Epstein-Bar virus (EBV), a member of the subfamily gammaherpesviruses that also includes the Kaposi Sarcoma-associated herpesvirus (KSHV),2,3 is the first identified oncovirus. Similar to other members of the family herpesviridae, EBV has a characteristic three-layer configuration: the outer lipid bilayer envelope containing viral glycoproteins responsible for host recognizing and membrane fusion, the inner pseudo-icosahedral nucleocapsid enclosing a 172-kb double-strand DNA (dsDNA) genome and the middle pleomorphic tegument compartment fulfilled with 20–40 different viral proteins. All herpesvirus capsid shell consists of 4 abundant proteins: the major capsid proteins (MCP) constituting the basic capsid skeleton through forming 150 hexons and 11 pentons, the small capsid proteins (SCP) binding to the tops of hexon MCPs or both hexon and penton MCPs, and the Tri1 and Tri2 forming the heterotrimeric triplexes to plug the large holes on the capsid floor. Once the viral dsDNA genome enters the procapsid shell through the portal that is located at a unique 5-fold vertex of the icosahedral capsid, the viral nucleocapsid is joined by the capsid-associated tegument complexes (CATCs).

We also determined the high-resolution structure of the CATC in portal-proximal penton vertices where the CATC binds exclusively to a specific one of the five registers. In order to do so, we performed focused 3D classification of the portal-proximal penton-vertex sub-particles (extracted from the C1 capsid) with a mask encompassing a region containing only one CATC. We finally obtained 93,334 (83.3%) CATC-binding portal-proximal penton vertex sub-particles. Through 3D refinement, we obtained reconstruction of the C1 CATC-binding portal-proximal penton vertex at 4.3 Å. The structure of CATC in the portal-proximal penton vertex is essentially identical to that in the portal vertex. Unlike its counterpart in KSHV that interacts with only one MCP,22 the head domain of BVRF1 simultaneously contacts two neighboring penton MCPs, mainly through the region of residues 291–314. As such, pORF64 (the BVRF1 homolog in KSHV) interacts with one penton MCP at the apex, whereas the head domain of EBV BVRF1 simultaneously contacts two neighboring MCPs at the middle of the MCP tower region. Each CATC binds both triplexes Ta and Tc. The interactions between the CATC and Ta are exclusively mediated by BGLF1. The interactions between the CATC and triplex Tc occur at the vertex-distal end of the CATC.

>MARRLPKPTLQGRLEADFPDSPLLPKFQELNQNNLPNDVFREAQRSYLVFLTSQFCYEEYVQRTFGVPRRQRAIDKRQRASVAGAGAHAHLGGSSATPVQQAQAAASAGTGALASSAPSTAVAQSATPSVSSSISSLRAATSGATAAASAAAAVDTGSGGGGQPHDTAPRGARKKQ[5x];>MKVQGSVDRRRLQRRIAGLLPPPARRLNISRGSEFTRDVRGLVEEHAQASSLSAAAVWRAGLLAPGEVAVAGGGSGGGSFSWSGWRPPVFGDFLIHASSFNNAEATGTPLFQFKQSDPFSGVDAVFTPLSLFILMNHGRGVAARVEAGGGLTRMANLLYDSPATLADLVPDFGRLVADRRFHNFITPVGPLVENIKSTYLNKITTVVHGPVVSKAIPRSTVKVTVPQEAFVDLDAWLSGGAGGGGGVCFVGGLGLQPCPADARLYVALTYEEAGPRFTFFQSSRGHCQIMNILRIYYSPSIMHRYAVVQPLHIEELTFGAVACLGTFSATDGWRRSAFNYRGSSLPVVEIDSFYSNVSDWEVIL[2x];>MDLKVVVSLSSRLYTDEIAKMQQRIGCILPLASTHGTQNVQGLGLGQVYSLETVPDYVSMYNYLSDCTLAVLDEVSVDSLILTKIVPGQTYAIKNKYQPFFQWHGTGSLSVMPPVFGREHATVKLESNDVDIVFPMVLPTPIAEEVLQKILLFNVYSRVVMQAPGNADMLDVHMHLGSVSYLGHHYELALPEVPGPLGLALLDNLSLYFCIMVTLLPRASMRLVRGLIRHEHHDLLNLFQEMVPDEIARIDLDDLSVADDLSRMRVMMTYLQSLASLFNLGPRLATAAYSQETLTATCWLR[4x];>MSNGDWGQSQRTRGTGPVRGIRTMDVNAPGGGSGGSALRILGTASCNQAHCKFGRFAGIQCVSNCVLYLVKSFLAGRPLTSRPELDEVLDEGARLDALMRQSGILKGHEMAQLTDVPSSVVLRGGGRVHIYRSAEIFGLVLFPAQIANSAVVQSLAEVLHGSYNGVAQFILYICDIYAGAIIIETDGSFYLFDPHCQKDAAPGTPAHVRVSTYAHDILQYVGAPGAQYTCVHLYFLPEAFETEDPRIFMLEHYGVYDFYEANGSGFDLVGPELVSSDGEAAGTPGADSSPPVMLPFERRIIPYNLRPLPSRSFTSDSFPAARYSPAKTNSPPSSPASAAPASAAPASAAPASAAPASAAPASAAPASAAPASAAPASSPPLFIPIPGLGHTPGVPAPSTPPRASSGAAPQTPKRKKGLGKDSPHKKPTSGRRLPLSSTTDTEDDQLPRTHVPPHRPPSAARLPPPVIPIPHQSPPASPTPHPAPVSTIAPSVTPSPRLPLQIPIPLPQAAPSNPKIPLTTPSPSPTAAAAPTTTTLSPPPTQQQPPQSAAPAPSPLLPQQQPTPSAAPAPSPLLPQQQPPPSAARAPSPLPPQQQPLPSATPAPPPAQQLPPSATTLEPEKNHPPAADRAGTEISPSPPFGQQPSFGDDASGGSGLVRYLSDLEEPFLSMSDSEEAESDLASDIPTTEDEDMFEDEVFSNSLESGSSAPTSPITLDTARSQYYQTTFDIETPEMDFVPLESNIARIAGHTYQEQAIVYDPASNREVPEADALSMIDYLLVTVVLEQGLIRSRDRSSVLNLLEFLKDWSGHLQVPTLDLEQLLTSELNIQNLANMLSENKGRAGEFHKHLAAKLEACLPSLATKDAVRVDAGAKMLAEIPQLAESDDGKFDLEAARRRLTDLLSGGDQEAGEGGGEPEDNSIYRGPHVDVPLVLDDESWKRLLSLAEAARTAVARQQAGVDEEDVRFLALLTAIEYGAPPAASVPPFVHNVAVRSKNAALHVRRCTADIRDKVASAASDYLSYLEDPSLPTVMDFDDLLTHLRHTCQIIASLPLLNIRYTSIEWDYRELLYLGTALSDMSGIPWPLERVEEDDPSIAPLPEFETVAKKQKELETTRENEKRLRTILDDIEAMLGLAGVASAPGAPISPASPSATPANHDNPEATPPLADTAALTIPVIEKYIANAGSIVGAAKNPTYIRLRDTIQQIVRSKKYLMNILKSITFYTIDNYIASFEESIDHLYRDLPVLDPEVQDGIDRILDPMVSEALHTFEMGNRLTLEPARLVALQNFATHSTLKETAAAVNLLPGLLAVYDATITGQAPEDALRLLSGLQNQLSQTLIPGKLKKRFLSYLQKLKNNNNDQLRQKEVQAWRLEAEGFKPATEEQLEAFLDTAPNKELKRQYEKKLRQLMETGRKEKEKLREQEDKERQERRAREANEAWARIRKALGARPEPAPTSPDDWNTLLASLLPDNTDSAAAAAAAVARNTDILDSLTQILAAMLLGITRVRRERLRSLLVDDGGAAERMEAAEPGWFTDIETGPLARLDAWPATPAATAKEGGGGRGAEEAAGALFRARTAADAIRSALAQTRQALQSPDMKSAVVNTDLEAPYAEYERGLAGLLEKRRAAEAALTAIVSEYVDRTLPEATNDPGQANLPPPPTIPQATAPPRLASDSALWPKKPQLLTRRERDDLLQATGDFFSELLTEAEAAEVRALEEQVRESQTLMAKAHEMAASTRRGFHTALEAVLSRSRDEAPDDELRSLLPSPPKAPVQAPLEAALARAAAGNGSWPYRKSLAAAKWIRGICEAVRGLSEGALALAGGAGAWLNLAAAADGEIHELTRLLEVEGMAQNSMDGMEELRLALATLDPKRVAGGKETVADWKRRLSRLEAIIQEAQEESQLQGTLQDLVTQARGHTDPRQLKIVVEAARGLALGASAGSQYALLKDKLLRYASAKQSFLAFYETAQPTVFVKHPLTNNLPLLITISAPPTGWGNGAPTRRAQFLAAAGPAKYAGTLWLETESPCDPLNPAYVSADTQEPLNYIPVYHNFLEYVMPTVLENPEAFSLTPAGRPQAIGPPQDDQERRRRTLASVASARLSAAAADSYWDTWPDVESNAGELLREYVSAPKALMEDLADNPIVAMTLLAHASLIASRNHPPYPAPATDREVILLEQREMMALLVGTHPAYAAAFLGAPSFYAGLGLVSALARDGGLGDLLSDSVLTYRLVRSPASGRGGMPSTTRGSNDGEDARRLTRHRIAGPPTGFIFFQDAWEEMDTRAALWPHPEFLGLVHNQSTARARACMLLLARRCFAPEALQQLWHSLRPLEGPVAFQDYLRDFVKQAYTRGEELPRAEGLEVPRETPSSYGTVTGRALRNLMPYGTPITGPKRGSGDTIPVSVFEAAVAAAFLGRPLTLFVSSQYLFNLKTLGQVRVVAPLLYCDGHSEPFRSLVETISLNFLQDLDGYSESFEPEMSIFARQAVWLRELLTEARAAKPKEARPPTVAILANRKNIIWKCFTYRHNLPDVQFYFNAAGASRWPTDVLNPSFYEHEDPPLPVGYQLPPNPRNVQELFSGFPPRVGHGLVSGDGFQSADNTPASSDRLQQLGGGETDQGEKGSTTAESEASGPPSPQSPLLEKVAPGRPRDWLSPTSSPRDVTVTPGLAAPITLPGPRLMARPYFGAETRASESPDRSPGSSPRPWPKDSLELLPQPAPQQPPSSPWASEQGPIVYTLSPHSTPSTASGSQKKHTIQIPGLVPSQKPSYPPSAPYKPGQSTGGIAPTPSAASLTTFGLQPQDTQASSQDPPYGHSIMQREKKQQGGREEAAEIRPSATRLPTAVGLRPRAPVVAAGAAASATPAFDPGEAPSGFPIPQAPALGSGLAAPAHTPVGALAPRPQKTQAQRPQDAAALPTPTIKAVGARPVPKATGALAAGARPRGQPTAAPPSAASPPRVSLPVRSRQQQSPAIPLPPMHSGSEPGARPEVRLSQYRHAGPQTYTVRKEAPPSAASQLPKMPKCKDSMYYPPSGSARYPAPFQALSFSQSVASPAPSSDQTTLLWNTPSVVTQFLSIEDIIREVVTGGSTSGDLVVPSGSPSSLSTAAPEQDLRYSLTLSQASRVLSRFVSQLRRKLERSTHRLIADLERLKFLYL[2x];> MDVHIDNQVLSGLGTPLLVHLFVPDTVMAELCPNRVPNCEGAWCQTLFSDRTGLTRVCRVFAARGMLPGRPSHRGTFTSVPVYCDEGLPELYNPFHVAALRFYDEGGLVGELQIYYLSLFEGAKRALTDGHLIREASGVQESAAAMQPIPIDPGPPGGAGIEHMPVAAAQVEHPKTYDLKQILLEITQEENRGEQRLGHAGSPALCLGLRLRAGAETKAAAETSVSKHHPALENPSNIRGSAGGEGGGGRAGTGGTVGVGSGALSRVPVSFSKTRRAIRESRALVRGIAHIFSPHALYVVTYPELSAQGRLHRMTAVTHASPATDLAEVSILGAPEREFRFLISVALRISASFREKLAMQAWTAQQEIPVVIPTSYSRIYKNSDLIREAFFTVQTRVSWESCWVKATISNAPKTPDACLWIDSHPLYEEGASAWGKVIDSRPPGGLVGAASQLVALGTDGHCVHLATTSDGQAFLVLPGGFVIKGQLALTPEERGYILARHGIRREQ;>[2x]MALSGHVLIDPARLPRDTGPELMWAPSLRNSLRVSPEALELAEREAERARSERWDRCAQVLKNRLLRVELDGIMRDHLARAEEIRQDLDAVVAFSDGLESMQVRSPSTGGRSAPAPPSPSPAQPFTRLTGNAQYAVSISPTDPPLMVAGSLAQTLLGNLYGNINQWVPSFGPWYRTMSANAMQRRVFPKQLRGNLNFTNSVSLKLMTEVVAVLEGTTQDFFSDVRHLPDLQAALILSVAYLLLQGGSSHQQRPLPASREELLELGPESLEKIIADLKAKSPGGNFMILTSGNKEARQSIAPLNRQAAYPPGTFADNKIYNLFVGAGLLPTTAALNVPGAAGRDRDLVYRIANQIFGEDVPPFSSHQWNLRVGLAALEALMLVYTLCETANLAEAATRRLHLSSLLPQAMQRRKPAMASAGMPGAYPVQTLFRHGELFRFIWAHYVRPTVAADPQASISSLFPGLVLLALELKLMDGQAPSHYAINLTGQKFDTLFEIINQKLLFHDPAAMLAARTQLRLAFEDGVGVALGRPSPMLAAREILERQFSASDDYDRLYFLTLGYLASPVAPS;>[5x]MASNEGVENRPFPYLTVDADLLSNLRQSAAEGLFHSFDLLVGKDAREAGIKFEVLLGVYTNAIQYVRFLETALAVSCVNTEFKDLSRMTDGKIQFRISVPTIAHGDGRRPSKQRTFIVVKNCHKHHISTEMELSMLDLEILHSIPETPVEYAEYVGAVKTVASALQFGVDALERGLINTVLSVKLRHAPPMFILQTLADPTFTERGFSKTVKSDLIAMFKRHLLEHSFFLDRAENMGSGFSQYVRSRLSEMVAAVSGESVLKGVSTYTTAKGGEPVGGVFIVTDNVLRQLLTFLGEEADNQIMGPSSYASFVVRGENLVTAVSYGRVMRTFEHFMARIVDSPEKAGSTKSDLPAVAAGVEDQPRVPISAAVIKLGNHAVAVESLQKMYNDTQSPYPLNRRMQYSYYFPVGLFMPNPKYTTSAAIKMLDNPTQQLPVEAWIVNKNNLLLAFNLQNALKVLCHPRLHTPAHTLNSLNAAPAPRDRRETYSLQHRRPNHMNVLVIVDEFYDNKYAAPVTDIALKCGLPTEDFLHPSNYDLLRLELHPLYDIYIGRDAGERARHRAVHRLMVGNLPTPLAPAAFQEARGQQFETATSLAHVVDQAVIETVQDTAYDTAYPAFFYVVEAMIHGFEEKFVMNVPLVSLCINTYWERSGRLAFVNSFSMIKFICRHLGNNAISKEAYSMYRKIYGELIALEQALMRLAGSDVVGDESVGQYVCALLDPNLLPPVAYTDIFTHLLTVSDRAPQIIIGNEVYADTLAAPQFIERVGNMDEMAAQFVALYGYRVNGDHDHDFRLHLGPYVDEGHADVLEKIFYYVFLPTCTNAHMCGLGVDFQHVAQTLAYNGPAFSHHFTRDEDILDNLENGTLRDLLEISDLRPTVGMIRDLSASFMTCPTFTRAVRVSVDNDVTQQLAPNPADKRTEQTVLVNGLVAFAFSERTRAVTQCLFHAIPFHMFYGDPRVAATMHQDVATFVMRNPQQRAVEAFNRPEQLFAEYREWHRSPMGKYAAECLPSLVSISGMTAMHIKMSPMAYIAQAKLKIHPGVAMTVVRTDEILSENILFSSRASTSMFIGTPNVSRREARVDAVTFEVHHEMASIDTGLSYSSTMTPARVAAITTDMGIHTQDFFSVFPAEAFGNQQVNDYIKAKVGAQRNGTLLRDPRTYLAGMTNVNGAPGLCHGQQATCEIIVTPVTADVAYFQKSNSPRGRAACVVSCENYNQEVAEGLIYDHSRPDAAYEYRSTVNPWASQLGSLGDIMYNSSYRQTAVPGLYSPCRAFFNKEELLRNNRGLYNMVNEYSQRLGGHPATSNTEVQFVVIAGTDVFLEQPCSFLQEAFPALSASSRALIDEFMSVKQTHAPIHYGHYIIEEVAPVRRILKFGNKVVF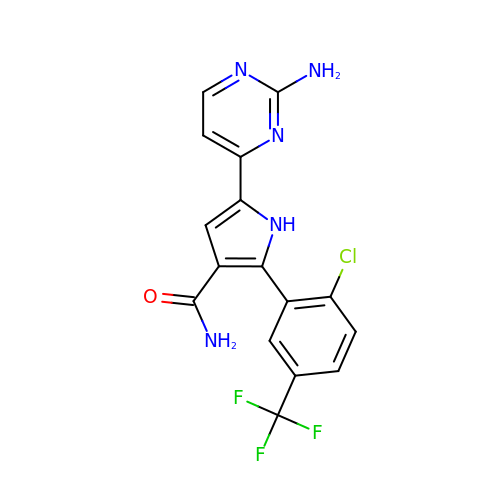5-(2-aminopyrimidin-4-yl)-2-[2-chloro-5-(trifluoromethyl)phenyl]-1H-pyrrole-3-carboxamide | C16 H11 Cl F3 N5 O | CZUQYAXYBOEHCY-UHFFFAOYSA-N>GAMDGTAAEPRPGAGSLQHAQPPPQPRKKRPEDFKFGKILGEGSFSTVVLARELATSREYAIKILEKRHIIKE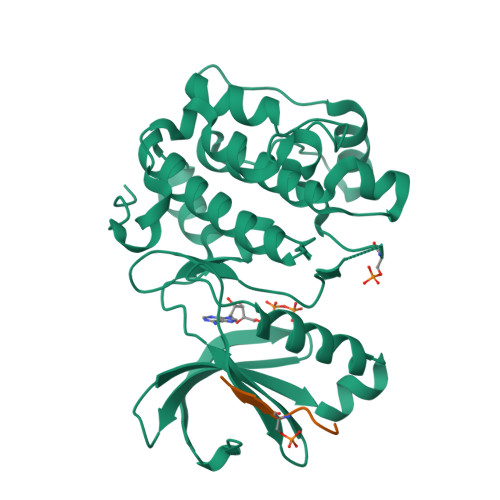NKVPYVTRERDVMSRLDHPFFVKLYFTFQDDEKLYFGLSYAKNGELLKYIRKIGSFDETCTRFYTAEIVSALEYLHGKGIIHRDLKPENILLNEDMHIQITDFGTAKVLSPESKQARANSFVGTAQYVSPELLTEKSACKSSDLWALGCIIYQLVAGLPPFRAGNEGLIFAKIIKLEYDFPEKFFPKARDLVEKLLVLDATKRLGCEEMEGYGPLKAHPFFESVTWENLHQQTPPKLT[4x];>KGAGGGGFPQFSYSA[4x]> MKKRLLLPLFAALCLSQIAHADEGMWLMQQLGRKYAQMKERGLKMKEYDLYNPNGTSLKDAVVLFDGGCTGEVVSDRGLVLTNHHCGYDMIQAHSTLEHNYLENGFWAMREADELPNKDISVVFIDKIEDVTDYVKKELKAIKDPNSMDYLSPKYLQKLADKKAGKNFSAKNPGLSVEIKAFYGGNLYLMFTKKTYTDVRLVGAPPSSIGKFGADTDNWIWPRHTGDFSIFRIYADKNGNPAPYSEDNVPLKPKRFFNISLGGVQENDYAMIMGFPGTTHRYFTASEVDEWKSIDNDIRIRMRDIRQGVMLREMLADPQIKIMYSAKYAASQNAYKRAIGAN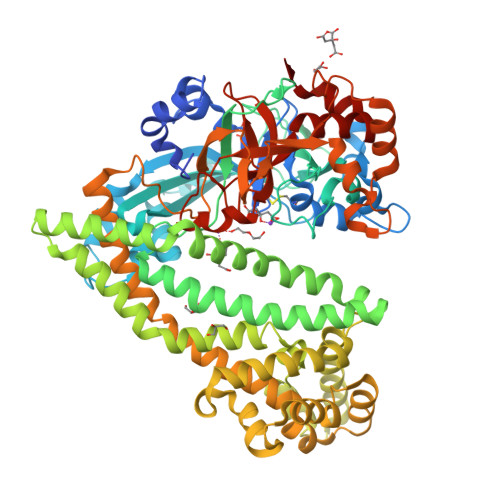WAIKTRGLRQNKQAMQDRLIAWGAKQGTPRYEEAVHEIDATVAKRADLRRRYWMIEEGIIRGIEFARSPIPTEDETKALQGNDASARKEAIDKIRTRYSKFANKDYSAEVDKKVAVAMLTEYLKEIPYENLPLHLRLVKDRFAGDVQAYVDDIFARSVFGSEAQFDAFAAVPSVEKLAEDPMVLFASSVFDEYRKLYNELRPYDDPILRAQRTYIAGLLEMDGDQDQFPDANLTLRFTYGQVKGYSPRDNVYYGHQTTLDGVMEKEDPDNWEFVVDPKLKAVYERKDFGRYADRSGRMPVAFCATTHTTGGNSGSPVMNANGELIGLNFDRNWEGVGGDIQYLADYQRSIIVDIRYVLLVIDKVGGCQRLLDEMNIVP> MKKEILKVERGSIAEELEIEKGDFLLSINNKEVKDIIDYKFLVCDEYLEVEIEKSNGELWELEIEKDYDEDLGIEFKAAILDVPQRCHNNCLFCFIDQLPKGMRKTLYFKDDDSRLSFLQGNFLTLTNMKDEDIERIINYKISPINISVHTTNPELRVELLNNRFAGNIYERMKKLAEGGIKMNCQVVLCPGLNNAEELKRTIEDLYALYPQVENLAVVPIGVTKFREGLYRFELFNKETANKELDMVEEYQNKFIKEIGKPFVRLSDEFYVIAEREIPKEEFYDGFHQLEDGVGVIRIFRNNIKNNVKKLSTKVKGSFSLITGQSAYKEILEASRIINNYNNDINIEVIKIDNNFFGKTITVAGLITANDIIEQTQEKNLGKYVIIPDVMLRKGYELADISEQVFLDDVTLKELSKSLKREILVCDYTGEDLIDIINKHSRE

Cobalamin (Cbl)-dependent radical S-adenosylmethionine (SAM) enzymes constitute a large subclass of radical SAM (RS) enzymes that use Cbl to catalyze various types of reactions, the most common of which are methylations. Bioinformatic analysis of Mmp10 identified DUF512 (Domain of Unknown Function 512) as a potential Cbl-binding domain in RS enzymes. X-ray crystal structures of DUF512-containing proteins from Clostridium sporogenes and Pyrococcus furiosus show unique architectural features and confirm the presence of a C-terminal Cbl-binding domain like that of Mmp10. We have uncovered the “Unknown Function” of the DUF512 protein domain, which is to bind the biological cofactor Cbl.

csDUF512 was crystallized under anoxic conditions in the presence of AzaSAM, and its structure was determined to a resolution of 1.68 Å. AzaSAM is a SAM analog containing a nitrogen atom in place of SAM’s sulfur atom, and it has been used as a SAM surrogate in several structural studies.19,42,43csDUF512 is composed of three domains (topology diagram in Figure S5A), the first of which (residues 1–80) is a PDZ domain. Of note, csDUF512 is the first structurally characterized RS enzyme with a PDZ domain. The second domain (residues 81–266) of csDUF512 has an unusually short and incomplete β3α4 TIM barrel core. Interestingly, csDUF512 lacks the starting strand (β1) in its RS domain. Instead, a short strand (β5) from the PDZ domain precedes the cluster-loop. Cys87, Cys91, and Cys94 coordinate the FeS cluster of csDUF512. Notably, an aspartate (D112) residue in the middle of a DDD motif located on the cluster loop is observed to coordinate the unique iron of the FeS cluster. The AzaSAM in the csDUF512 structure shows a very different binding pose compared to SAM in the Mmp10 structure.21 Some of the canonical motifs for SAM binding, such as a Glu residue interacting with the ribose moiety of SAM and the GXIXGXXE motif, are not observed. After rotation, the adenosine moiety remains in the same position, but the methyl group of AzaSAM is significantly closer to the cobalt ion.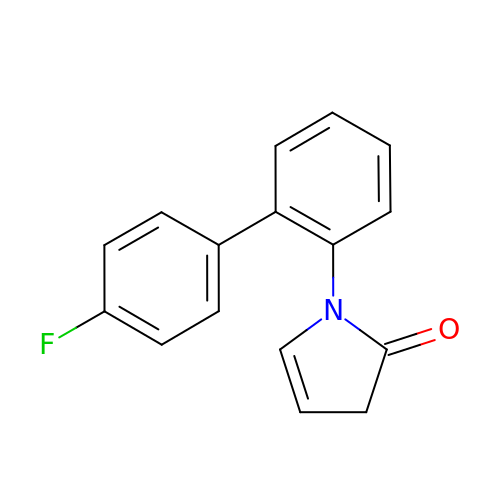1-(4'-fluoro[1,1'-biphenyl]-2-yl)-1,3-dihydro-2H-pyrrol-2-one | C16 H12 F N O | XQHVGZKJQZFCRP-UHFFFAOYSA-N>[2x]MIRYPNGKTFQPKHSVSSQNSQKRAPSYSNRGMTLEDDLNETNKYYLTNQIAVIHKKPTPVQI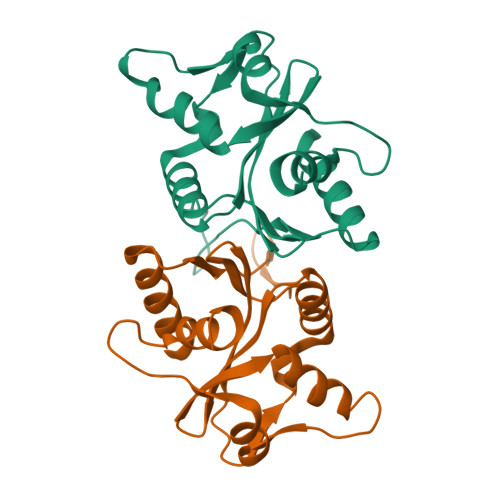VNVHYPKRSAAVIKEAYFKQSSTTDYNGIYKGRYIDFEAKETKNKTSFPLQNFHDHQIEHMKQVKAQDGICFVIISAFDQVYFLEADKLFYFWDRKEKNGRKSIRKDELEETAYPISLGYAPRIDYISIIEQLYFSPSSGAKG>SNAMKTNDNYIE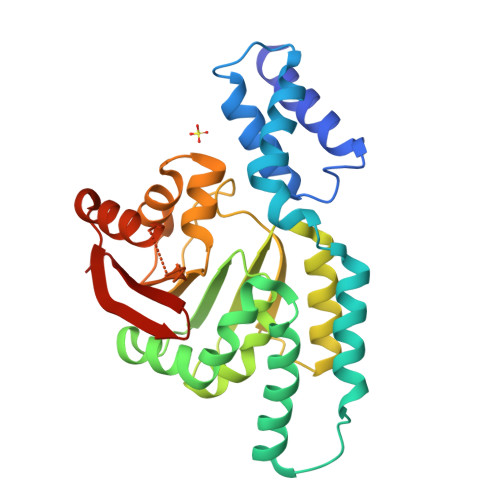EVTAKVLTSGKYSTLYPPTVRRVTERLFDRYPPKQLEKEVRKKLHQAYGAYIGGIDGKRLEKKIEKIIHEIPNPTTDEATRTEWEKEICLKILNLHTSTNERTVAYDELYQKIFEVTGVPTSITDAGCALNPFSFPFFTEAGMLGQYIGFDLDKGMIEAIEHSLRTLNAPEGIVVKQGDILSDPSGESDLLLMFKLYTLLDRQEEASGLKILQEWKYKNAVISFPIKTISGRDVGMEENYTVKFENDLVGSDLRIMQKLKLGNEMYFIVSRL[4x]>MEMRVLLIAGGVSPEHEVSLLSAEGVLR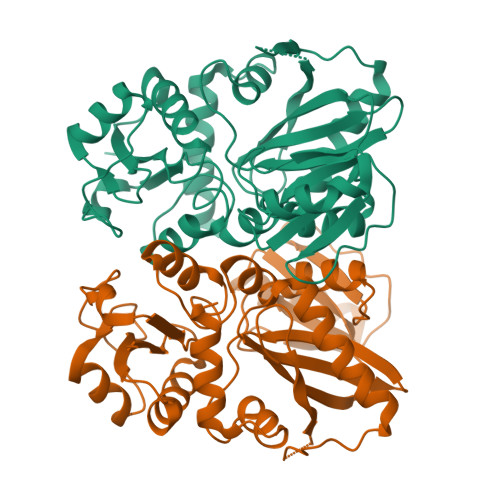HIPFPTDLAVIAQDGRWLLGEKALTALEAKAAPEGEHPFPPPLSWERYDVVFPLLHGRFGEDGTVQGFLELLGKPYVGAGVAASALCMDKDLSKRVLAQAGVPVVPWVAVRKGEPPVVPFDPPFFVKPANTGSSVGISRVERFQDLEAALALAFRYDEKAVVEKALSPVRELEVGVLGNVFGEASPVGEVRYEAPFYDYETKYTPGRAELLIPAPLDPGTQETVQELALKAYKVLGVRGMARVDFFLAEGELYLNELNTIPGFTPTSMYPRLFEAGGVAYPELLRRLVELALTHHHHHH[4x]Here, crystal structures of human NLRP14 pyrin-domain variants are reported. Structurally, NLRPs share a conserved tripartite domain architecture consisting of an N-terminal pyrin domain, a central NACHT domain (with reference to its initial identification in NAIP, CIITA, Het-E and TP1) and a C-terminal leucine-rich repeat (LRR) domain. Pyrin domains belong to the death-domain superfamily, which includes the CARDs, the death-effector domains (DEDs) and the death domains (DDs) in addition to the PYDs. The death-domain fold consists of six antiparallel α-helices packed around a highly conserved hydrophobic core with Greek-key topology.

NLRP14 PYD contains Leu at the central position 84, thereby breaking the charge bridge. To test the relevance of the proposed charge bridge to the pyrin-domain conformation, we introduced a L84R mutant to reconstitute the stabilizing charge bridge. The introduced positive charge of Arg84 bridges the negative charges of the opposing Glu26 and Asp86. This structure further confirms the proposed adaptive role of the hydrophobic residues Trp72, Leu76 and Leu87 that contribute to the hydrophobic core and thereby stabilize helix α6 within the bundle. With this crystal structure analysis we have identified a conformational regulation element (CRE) that allows us to predict the tendency of pyrin domains to adopt the closed or open conformation. Our previous structure-derived conclusions on the significance of the charge bridge/CRE suggested that the L84R mutant should adopt a stable six-helix bundle conformation. The L84R variant adopts a canonical death-domain fold with all six helices contributing to the stabilizing hydrophobic core. In quantitative terms, the hydrophobic core in the canonical six-helix bundle form (L84R) amounts to 2435 Å2, whereas the corresponding contact area will be reduced in the wild-type protein by approximately 490 Å2 to 1945 Å2, i.e. an approximate 20% reduction in the stabilizing interaction interface. By contrast, the L84R mutant crystallized in space group P21212 with one (monomeric) molecule per asymmetric unit. While the engineered L84R mutant showed remarkable properties such as a drastically improved thermal stability that correlates with a strictly monomeric six-α-helix structure, the naturally occurring D86V mutant behaved very much like the wild-type protein despite its severe physiological implications.

> GSHMADSSSSSFFPDFGLLLYLEELNKEELNTFKLFLKETMEPEHGLTPWNEVKKARREDLANLMKKYYPGEKAWSVSLKIFGKMNRKDLCERAKEEINWSAQLE> LENKPRIPVVWIHGLECTCCTESFIRSAHPLAKDVILSLISLDYDDTLMAAAGTQAEEVFEDIITQYNGKYILAVEGNPPLGEQGMFCISSGRPFIEKLKRAAAGASAIIAWGTCASWGCVQAA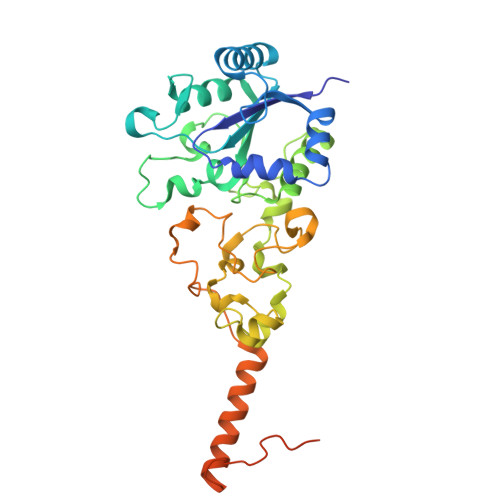RPNPTQATPIDKVITDKPIIKVPGCPPIPDVMSAIITYMVTFDRLPDVDRMGRPLMFYGQRIHDKCYRRAHFDAGEFVQSWDDDAARKGYCLYKMGCKGPTTYNACSSTRWNDGVSFCIQSGHGCLGCAENGFWDRGSFYSRVVDIPQMGTHSTADTVGLTALGVVAAAVGVHAVASAVDQRRRHNQQPTETEHQPGNEDKQARSHHHHHH> MTEAPDVDLADGNFYASREARAAYRWMRANQPVFRDRNGLAAASTYQAVIDAERQ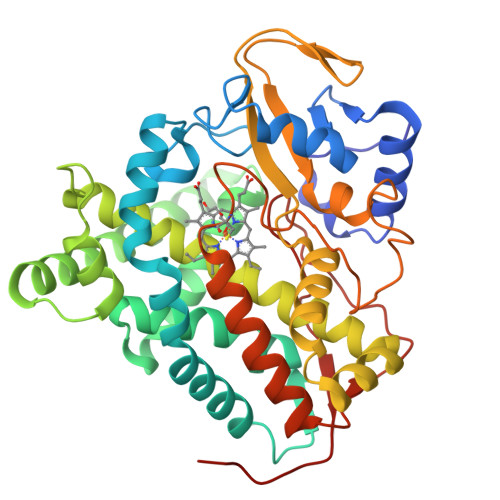PELFSNAGGIRPDQPALPMMIDMDDPAHLLRRKLVNAGFTRKRVKDKEASIAALCDTLIDAVCERGECDFVRDLAAPLPMAVIGDMLGVRPEQRDMFLRWSDDLVTFLSSHVSQEDFQITMDAFAAYNDFTRATIAARRADPTDDLVSVLVSSEVDGERLSDDELVMETLLILIGGDETTRHTLSGGTEQLLRNRDQWDLLQRDPSLLPGAIEEMLRWTAPVKNMCRVLTADTEFHGTALCAGEKMMLLFESANFDEAVFCEPEKFDVQRNPNSHLAFGFGTHFCLGNQLARLELSLMTERVLRRLPDLRLVADDSVLPLRPANFVSGLESMPVVFTPSPPLG> MTDTARLRAILAAHRGREGALLPILHDVQAAFGFIPEDAYAPIAADLGLTRAEVAGVVGFYHDFRKAPAG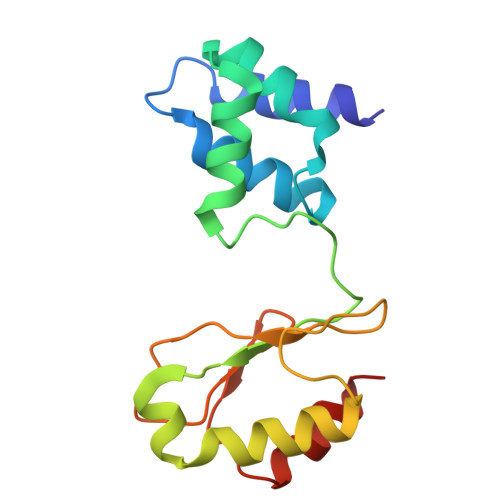RHVIKLCRAEACQAMGMDAVQARLESALGLRLGDSSEAVTLEAVYCLGLCACAPAAMVDDRLVGRLDAAAVAGIVAELGA>[8x]GVSGHRDMIST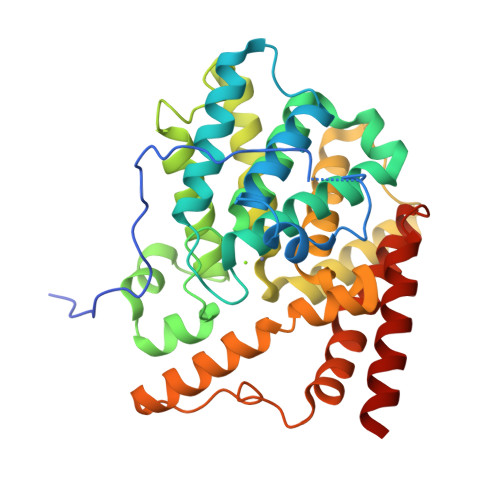RRLPPSIVQDTILAVVPPKSCAAIGTDVDLRDWGFDTFEVASRVPSVLQSVAMHVALAWDFFASQEEAQKWAFLVAAVENNYRPNPYHNAIHAADVLQGTFSLVSAAKPLMEHLTPLECKAAAFAALTHDVCHPGRTNAFLAAVQDPVSFKFSGKGTLEQLHTATAFELLNVTEFDFTSSMDNASFLEFKNIVSHLIGHTDMSLHSETVAKHGAKLSAGGFDCTCKEDRLEALSLLLHAADIGASSRGVAIARKWLVILQEFADQAEDERRRGLPVTPGFETPSSVEKSQIPFLDFFVIPTFDLLHQLFPSIEEPLHNLRKLRELYAAKAGVTT> MTQAWLWIGVISMALGSVFFGFGAHNAKNERWQILYTLNFFICLIAA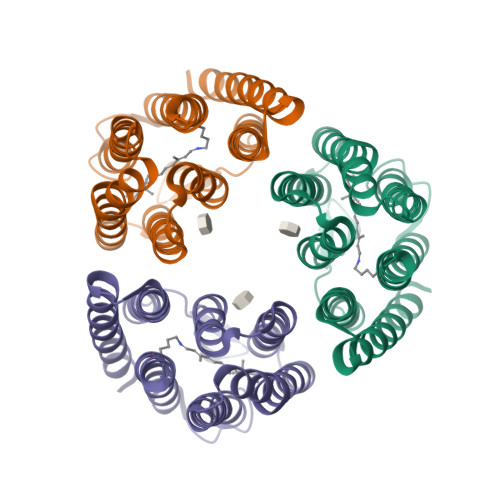GLYLAMALGLGVNVINGRPTYWVRFVDWFCSTPLLLLDLTFLGRTSLPLTGSLLGANAYMLVTGFVATVTPKPMSYIWYIVSCAAYLAIVYLLAQPYRIAAERKHPRSKQAFRTLVTVHLVLWTLYPIVWILSPEGFSTFTQGSETMFYTLLDIASKVGFGFLSLNTLHTLEQATEPARETHLSYLEHHHHHH Vertebrate type-IIa RPTPs comprise LAR, PTPσ and PTPδ, which share common domain architecture with a single transmembrane (TM) helix flanked by a large extracellular domain (ECD) and cytoplasmic tandem PTP domains: the membrane-proximal PTP domain (D1) is catalytically active, whereas the membrane-distal PTP domain (D2) is inactive. In mammals, presynaptic type-IIa RPTPs form trans-synaptic adhesion by specifically binding to their cognate postsynaptic organizers through their ECDs for inducing synaptic differentiation of neurons. To date, five different types of postsynaptic organizers for type-IIa RPTPs have been reported: interleukin-1 receptor (IL-1R) accessory protein (IL-1RAcP)7, IL-1RAcP-like-1 (IL1RAPL1)8, neurotrophin receptor tyrosine kinase C (TrkC), netrin-G ligand-3 (NGL-3)1011 and Slit- and Trk-like (Slitrk) family proteins. To elucidate the structural basis for decoding the ‘splice-insert signaling code' in the type-IIa RPTPs, we determined the crystal structures of PTPδ-ECD in complex with IL-1RAcP-ECD and IL1RAPL1-ECD.

To elucidate the structural basis of the PTPδ–IL1RAPL1 interaction for trans-synaptic adhesion, we determined the crystal structures of IL1RAPL1-ECD in complex with PTPδ Ig1-Ig2 and the full-length PTPδ-ECD at 2.7 and 4.4 Å resolutions, respectively. Description of PTPδ Ig1-Ig2 will be based on the 2.7-Å-complex structure, whereas that of the other regions of PTPδ-ECD will be based on the 4.4-Å-complex structure. The Ig1-Ig2 domains of PTPδ retain the binding ability for IL1RAPL1-ECD, as shown in our serial deletion analysis of PTPδ. No substantial change in the backbone structure of PTPδ Ig1-Ig2 occurred upon binding to IL1RAPL1. The interface between the IL1RAPL Ig1 and PTPδ Ig2 domains comprises both hydrophobic and hydrophilic interactions with a buried surface area of 699 Å2. These interactions occur on two β-strands comprising Arg181–Ser187 and Arg196–Glu202 in the Ig2 domain of PTPδ, between which meA9 is inserted. The first eight residues of meA9 (188Glu-Ser-Ile-Gly-Gly-Thr-Pro-Ile195) form a loop connecting these two β-strands, whereas the last residue, Arg196, extends one of the two β-strands. Trp34 of IL1RAPL1 hydrophobically interacts with Leu153, Ala198 and Leu185 of PTPδ. The Arg196 side chain forms a hydrogen bond with Asp37 of IL1RAPL1, which is further stabilized by a hydrogen bond with Tyr59 of IL1RAPL1. The IL1RAPL1 Ig3–PTPδ Ig1 interface is overlapped with the putative binding pocket for glycosaminoglycan chains of heparan sulfate and chondroitin sulfate proteoglycans, which mediate axonal growth control though the interaction with the type-IIa RPTPs19. This third interface is formed primarily by hydrophilic interactions: a positively charged cluster comprising Arg75, Arg95 and Arg98 of PTPδ forms a hydrogen bond network with a negatively charged cluster comprising Glu291 and Asp292 of IL1RAPL1.

> ETPPRFTRTPVDQTGVSGGVASFICQATGDPRPKIVWNKKGKKVSNQRFEVIEFDDGSGSVLRIQPLRTPRDEAIYECVASNNVGEISVSTRLTVLREDQIPRGFPTIDMGPQLKVVERTRTATMLCAASGNPDPEITWFKDFLPVDTSNNNGRIKQLRSESIGGTPIRGALQIEQSEESDQGKYECVATNSAGTRYSAPANLYVRELREVRRVPPRFSIPPTNHEIMPGGSVNITCVAVGSPMPYVKWMLGAEDLTPEDDMPIGRNVLELNDVRQSANYTCVAMSTLGVIEAIAQITKHHHHHH;> PAARDLKVVTKRGSADGCTDWSVDIKKYQVLVGEPVRIKCALFYGYIRTNYSLAQSAGLSLMWYKSSGPGDFEEPIAFDGSRMSKEEDSIWFRPTLLQDSGLYACVIRNSTYCMKVSISLTVGENDTGLCYNSKMKYFEKAELSKSKEISCRDIEDFLLPTREPEILWYKECRTKAWRPSIVFKRDTLLIKEVKEDDIGNYTCELKYGGFVVRRTTELTVTAPLTDKPPKLLYPMESKLTVQETQLGGSANLTCRAFFGYSGDVSPLIYWMKGEKFIEDLDENRVWESDIRILKEHLGEQEVSISLIVDSVEEGDLGNYSCYVENGNGRRHASVLLHKRKHHHHHH>[12x]MAIPKIASYSIPLAETFPKNKVHWHVQADRAVLLIHDMQKYFINFFDHSQAPVPELLANISELKSLA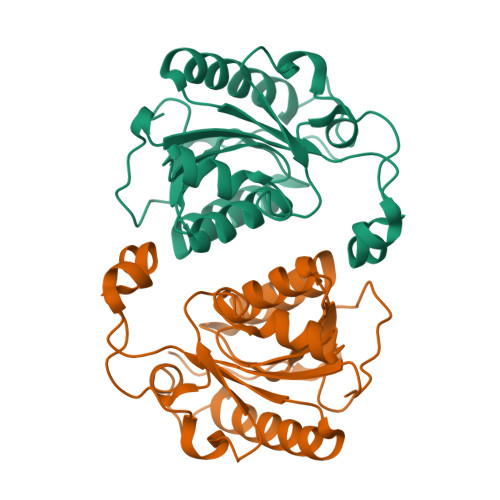RQANIPVVYTAQPPNQDPIERALLTDFWGTGLTKDTEIVSELSPEDGDIQYTKWRYSAFKKTPLLERMKETQRDQLIIVGVYAHIGILSTALDAFMLDIQPFVVGDAVADFSLEDHHHTLKYITERVGCVTSLEALKPQMIHSQETRLLS Inositol pyrophosphates (PP-InsPs) are eukaryotic nutrient messengers. The N-terminal kinase domain of diphosphoinositol pentakisphosphate kinase (PPIP5K) generates the messenger 1,5-InsP8, the C-terminal phosphatase domain catalyzes PP-InsP breakdown. The balance between kinase and phosphatase activities regulates 1,5-InsP8 levels. ScVip1PD is a phytase-like inositol 1-pyrophosphate histidine phosphatase with two conserved catalytic motifs.

Next, we replaced the catalytic loop residues Arg547, His548 and Arg551 in ScVip1PD Δ848-918 with alanine and obtained crystals in complex with the substrate 1,5-InsP8 diffracting at ~2.4 Å resolution (ScVip1PD Δ848-918 RHR-AAA). Notably, the GAF domain adopts a “closed” conformation in the substrate-bound structure. In our ScVip1PD Δ848-918 RHR-AAA—1,5-InsP8 complex structure, we located a crystallographic dimer stabilized by an intermolecular disulfide bridge involving a cysteine (Cys793) that, in apo structures, is part of the zinc-binding site. One molecule of 1,5-InsP8 is bound to each monomer, either on the surface of the enzyme involving the GAF domain or near the catalytic center. The GAF domain adopts a closed conformation in both monomers. In both binding sites, all phosphate groups of 1,5-InsP8 are well defined by electron density, with the 1-β-phosphate facing away from the active site. Conserved basic residues from the GAF domain and the α-insertion domain contribute to the formation of the outer substrate binding surface. A large network of lysine residues from the GAF domain and from the base of the α-insertion domain forms the second substrate binding surface, which is located in close proximity to the RHxxR catalytic loop. Most of the basic residues contributing to the outer and the inner 1,5-InsP8 binding surfaces map to the central β-sheet of the GAF domain. Comparison of the outer and inner substrate binding sites in ScVip1PD suggests that the 1,5-InsP8 substrate may undergo a ~90° rotation upon entering the active site.

>[2x]GAKWVFKGLAIIIAAADATPKQKFKHSFTSPIFISLLKGHKEEVVIRNVNDLKIVLQALRIALDEKAGNPAKIKVLANALEKKLNFPGTKIQLKPVLNKENEVEKVQFILKWGGEPTHSAKYQATELGEQMRQDFDLLNKSILQNIKIFSSSERRVLHTAQYWTRALFGADELGSDEISIRKDLLDDSNAAKDLMDKVKKKLKPLLREGKEAPPQFAWPSKMPEPYLVIKRVVELMNYHKKIMDNNFAKKDVNSMQTRWCTSEDPSLFKERWDKLFKEFNNAEKVDPSKISELYDTMKYDALHNRQFLENIFDPGSSGQFDEPRFMQLRELYKLAKVLFDFICPKEYGISDAEKLDIGLLTSLPLAKQILNDIGDMKNRETPACVAYFTKESHIYTLLNIIYESGIPMRIARNALPELDYLSQITFELYESTDASGQKSHSIRLKMSPGCHTQDPLDVQLDDRHYISCIPKISLTKHLDMDYVQQKLRNKFTRVIMPPKFTPVNITS> GGSGQTQPLKSVFSIDAGRKYFSVEQLEELVAKASQNGYTDVQLILGNDGLRFILD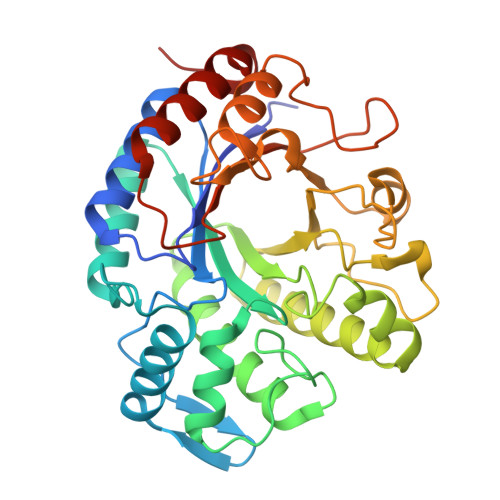DMSVNVNGKKYNHNRVSKAIQRGNNAYYNDPNGNALTQKEMDRLLAFAKARNINIIPVINSPGHMDALLVAMEKLAIKNPAFDGSKRTVDLGNQKAVNFTKAIISKYVAYFSAHSEIFNFGGDEYANDVDTGGWAKLQSSGRYKDFVAYANDLAKIIKDAGMQPMSFNDGIYYNSDDSFGTFDPEIIISYWTAGWSGYDVAKPEYFVQKGHKIFNTNDAWYWVAGNVDSGIYQYDDALANMSKKAFTDVPAGSPNLPIIGSIQCVWYDDPRRDYDFERIYTLMDTFSENYREYMVVKNH>[3x]MRGSHHHHHHGRSLNPLSTPQFDSTDETPASYNLAVRRAAPAVVNVYNRGLNTNSHNQLEIRTLGSGVIMDQRGYIITNKHVINDADQIIVALQDGRVFEALLVGSDSLTDLAVLKINATGGLPTIPINARRVPHIGDVVLAIGNPYNLGQTITQGIISATGRIGLNPTGRQNFLQTDASINPGNSGGALVNSLGELMGINTLSFDKSNDGETPEG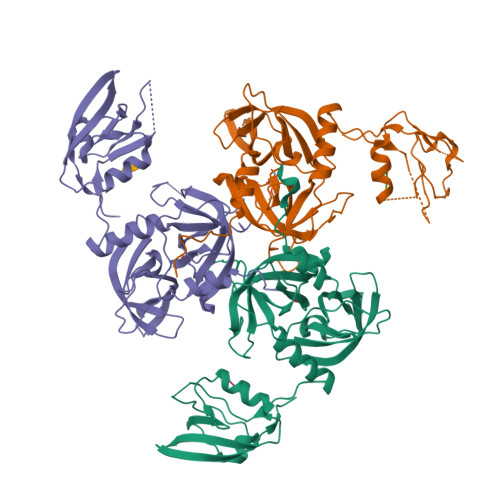IGFAIPFQLATKIMDKLIRDGRVIRGYIGIGGREIAPLHAQGGGIDQLQGIVVNEVSPDGPAANAGIQVNDLIISVDNKPAISALETMAQVAEIRPGSVIPVVVMRDDKQLTLQVTIQEYPATN;>[3x]YRF1-amino-5-(5-hydroxy-2-methylphenyl)-7,8,9,10-tetrahydropyrimido[4,5-c]isoquinolin-6(5H)-one | C18 H18 N4 O2 | 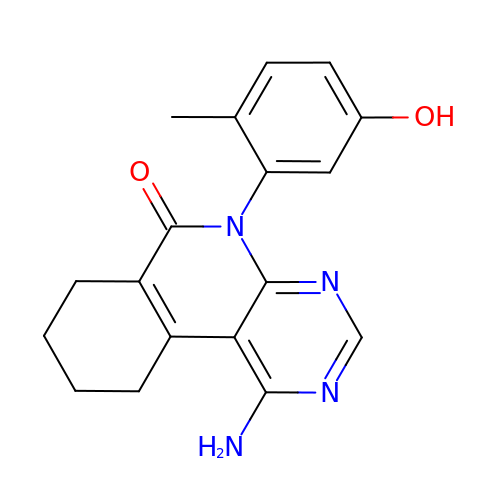ZQQZSFIPDUAFMC-UHFFFAOYSA-N UDP-2-acetamido-4-amino-2,4,6-trideoxy-alpha-D-glucopyranose | C17 H28 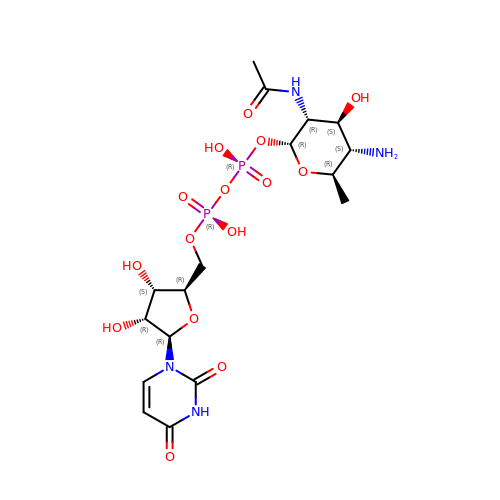N4 O15 P2 | FUUMLYWEEZBCQR-UINYWEPJSA-N>[3x]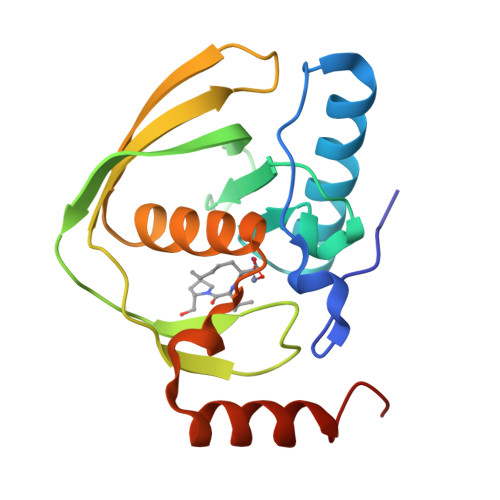SVLQVLHIPDERLRKVAKPVEEVNAEIQRIVDDMFETMYAEEGIGLAATQVDIHQRIIVIDVSENRDERLVLINPELLEKSGETGIEEGCLSIPEQRALVPRAEKVKIRALDRDGKPFELEADGLLAICIQHEMDHLVGKLFMDYLSPLKQQRIRQKVEKLDRLKARA> AYQDPGRLGAPDSWKTAEFNRQWGLEAISAEFAYARGYTGKGITIGVIDNAILSHSEFSGKLTRLDNGSYNFSYDKQDNMSFGDHGT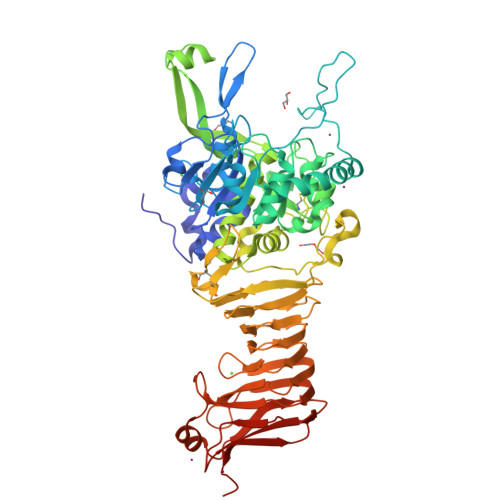HVAGIAAAKRDGAGMHGVAFDADIIGTKLNDYGNRNGREELIQSAARVINNSWGIAPDIRRDAKGDIIWLPNGRPDYVAFVKSEVIAEMMRSKSSVEWGSEQPVPTGGHSAMSTLLRAARHGKLIVFSAGNYNNYNIPEAQKSLPYAFPDVLNNYLIVTNLSDENQLSVSSTSCGQTASYCVSAPGSDIYSTVGRLESNTGGAVNREAYNKGELSLNPGYGNKSGTSMAAPHVTGVAAVLMQRFPYMSADQISAVIKTTATDLGVAGIDNLFGWGRVNLRDAINGPKMFITKEDIPQEYYVPGSYSEKQFVVNIPGLGNIVEPGTPVERRCTSSECSFDSWSNDISGHGGLTKTGAGTLALLGNNTYRGDTWVKQGVLAIDGSVASNVYIENSGTLSGEGTVGAFRAARSGSVAPGNGIGTLHVLHDAIFDRGSQYNVEVADNGRSDKIAARRAFLNGGSVNVSLERSQNLLSQNEAQSLLGNKYTILTTTDGVTGRFENANPSYPFVKVALDYRGNDVGLGITRTDASFD>THLNTYESVTPDPDVDVIIIGAGISGSAAAKALHDQGASVLVVEANDRIGGRTWTEQEGAPGGPIDYGGMFIGETHTHLIELGTSLGLEMTPSGKPGDDTYIVAGNVLRAPDDQLD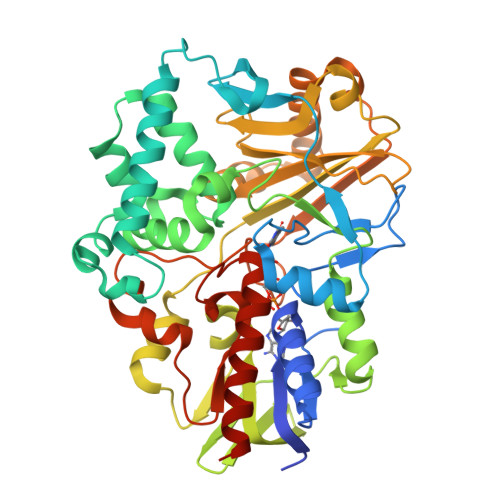PNLPFVPEFLSSLKALDELADSVGWDQPWASPNAAALDSKTVATWLAETIESEEVRRLHTVIVNTLLGADPYEVSLLYWAYYVSECEGIQSLMGTRDGAQWAWWFGGAAQVSWRIADAIGRDKFLLEWPVDRIEHDESGVTLFSGQRSLRARHIVIAMSPLAANQIRFEPALPTSRAQLQARAPMGRYYKVQARYPSSFWVEQGYSGALLDTEDVGVFLLDGTKPTDTLATLIGFIGGSNYDRWAAHTPQERERAFLDLLVKAFGPQAADPSYFHETDWTQQEWAKGGPVTYMPPGVLANFGAALRDPVGKVHFAGTEASFQWSGYMEGGVRAGQKAAAAIAEELERTANKGALV[4x]~{S}-[2-[3-[[(2~{R})-4-[[[(2~{R},3~{S},4~{R},5~{R})-5-(6-aminopurin-9-yl)-4-oxidanyl-3-phosphonooxy-oxolan-2-yl]methoxy-oxidanyl-phosphoryl]oxy-oxidanyl-phosphoryl]oxy-3,3-dimethyl-2-oxidanyl-butanoyl]amino]propanoylamino]ethyl] 2-(2,5-dihydrooxepin-7-yl)ethanethioate | C29 H44 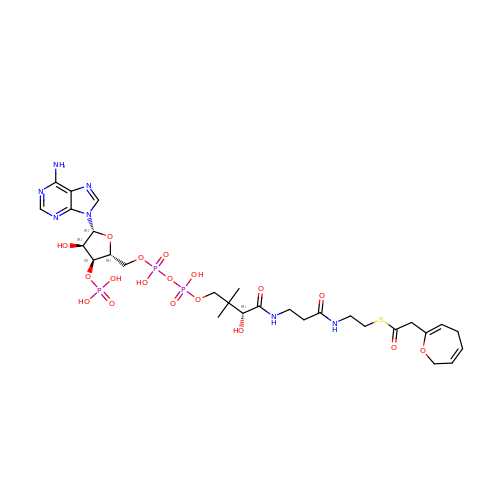N7 O18 P3 S | GQJGZLQATBGDEV-CECATXLMSA-N Escherichia coli phage SU10 belongs to the genus Kuravirus from the class Caudoviricetes of phages with short non-contractile tails. Here we show that the virion of SU10 has a prolate head, containing genome and ejection proteins, and a tail, which is formed of portal, adaptor, nozzle, and tail needle proteins and decorated with long and short fibers. In contrast to other short-tailed phages, the tails of Kuraviruses elongate upon cell attachment. After binding to the host, SU10 tail, nozzle proteins, and short fibers re-arrange to form a nozzle that extends the tail.

The prolate capsid of SU10 is organized with fivefold symmetry and is built from 715 copies of the major capsid protein organized with the triangulation parameters Tend = 4, Tmid = 20. The major capsid protein forms capsomers of two types: pentamers and hexamers. The closure of the caps is enabled by pentamers, which are bent in contrast to the flatter hexamers. However, the formation of the prolate SU10 head also requires variation in the shape of hexamers and in the angles at which they interact. The major capsid protein of SU10 has an HK97 fold, which is common among tailed bacteriophages and herpesviruses. According to the convention, the capsid protein can be divided into the N-terminal arm, peripheral domain, extended loop, axial domain, and glycine-rich loop. The major difference between the capsid proteins forming hexamers and pentamers is in the structure of the annular loop positioned at the tip of the axial domain. The capsid of the genome release intermediate of SU10 is identical to that of the virion.

>MANPTLFVSYDQNGKKLSFANWISVLSPQDTPFVSMTGKESINQTIFSWQTDALASVDGNNAHVEGSRAEDGEMKPTVIKSNVTQILRKVVRVSDTANTTANYGRGRELMYQLEKKGKEIKRDLEKILLSGQARTDVLADQYLTNSAADPAVAGLNDTHAARKTGAFQFLCAHGGLAGGVVDKTKNGPADPDTGAVTVKVAQNASNPTTNIGFDEADIFDMTLQLYTAGSEADIIMINPAHAKIFAGLQENTQGSRKRIFENTKQFIYEVNSITDPLGQSYKIIVNRWMPTDAVYFFRSADWTQMVLRAPKRTELAKDGSYEKWMIEMEVGLRHRNPYASGVLFTAAGKAAA[95x]> ATPSMMPQWSYMHISGQDASEYLSPGLVQFARATETYFSLNNKFRNPTVAPTHDVTTDRSQRLTLRFIPVDREDTAYSYKARFTLAVGDNRVLDMASTYFDIRGVLDRGPTFKPYSGTAYNALAPKGAPNSCEWEQTEDSGRAVAEDEEEEDEDEEEEEEEQNARDQATKKTHVYAQAPLSGETITKSGLQIGSDNAETQAKPVYADPSYQPEPQIGESQWNEADANAAGGRVLKKTTPMKPCYGSYARPTNPFGGQSVLVPDEKGVPLPKVDLQFFSNTTSLNDRQGNATKPKVVLYSEDVNMETPDTHLSYKPGKGDENSKAMLGQQSMPNRPNYIAFRDNFIGLMYYNSTGNMGVLAGQASQLNAVVDLQDRNTELSYQLLLDSIGDRTRYFSMWNQAVDSYDPDVRIIENHGTEDELPNYCFPLGGIGVTDTYQAIKANGNGSGDNGDTTWTKDETFATRNEIGVGNNFAMEINLNANLWRNFLYSNIALYLPDKLKYNPTNVEISDNPNTYDYMNKRVVAPGLVDCYINLGARWSLDYMDNVNPFNHHRNAGLRYRSMLLGNGRYVPFHIQVPQKFFAIKNLLLLPGSYTYEWNFRKDVNMVLQSSLGNDLRVDGASIKFDSICLYATFFPMAHNTASTLEAMLRNDTNDQSFNDYLSAANMLYPIPANATNVPISIPSRNWAAFRGWAFTRLKTKETPSLGSGYDPYYTY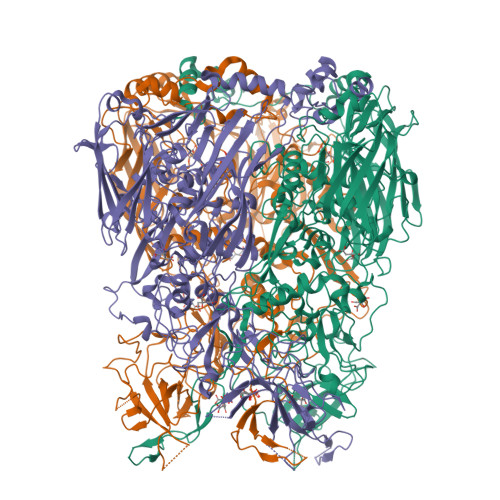SGSIPYLDGTFYLNHTFKKVAITFDSSVSWPGNDRLLTPNEFEIKRSVDGEGYNVAQCNMTKDWFLVQMLANYNIGYQGFYIPESYKDRMYSFFRNFQPMSRQVVDDTKYKEYQQVGILHQHNNSGFVGYLAPTMREGQAYPANVPYPLIGKTAVDSITQKKFLCDRTLWRIPFSSNFMSMGALTDLGQNLLYANSAHALDMTFEVDPMDEPTLLYVLFEVFDVVRVHQPHRGVIETVYLRTPFSAGNATT(3aR,5aS,8S,10aS)-1-[(3S,6R,8aS)-1'-[(2S)-2-acetamido-3-(2-chlorophenyl)propanoyl]-5-oxidanylidene-spiro[1,2,3,8a-tetrahydroindolizine-6,2'-pyrrolidine]-3-yl]carbonyl-10-oxidanylidene-2,3,3a,5a,8,10a-hexahydrodipyrrolo[3,2-b:3',1'-f]azepine-8-carboxylic 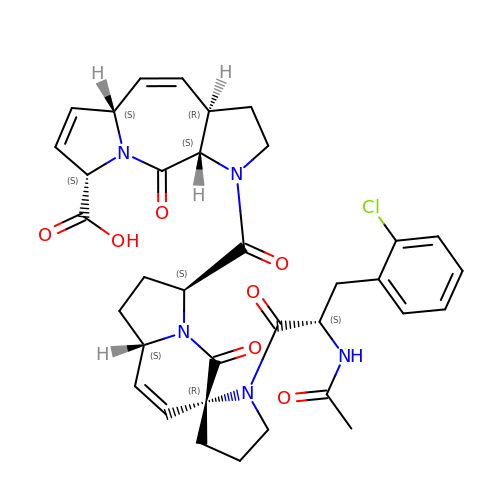acid | C35 H38 Cl N5 O7 | PORJLWGURWUCLW-QHVDBZGRSA-N6-amino-2-(methylamino)-4-(4-(trifluoromethyl)phenethyl)-3,7-dihydro-8H-imidazo[4,5-g]quinazolin-8-one 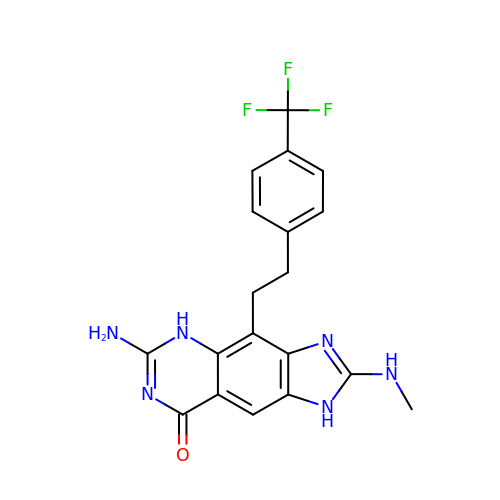| C19 H17 F3 N6 O | ZWUPQNLDYYEWTK-UHFFFAOYSA-N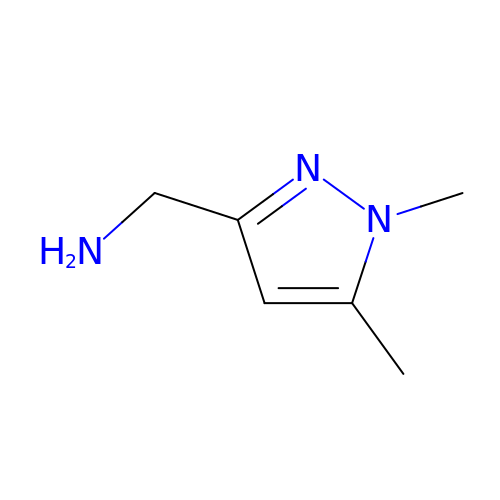1-(1,5-dimethyl-1H-pyrazol-3-yl)methanamine | C6 H11 N3 | JGYXJOBBROGMLL-UHFFFAOYSA-N>[6x]TLGTGNNGAKTEINKDGLTITPANGAGANNANTISVTKDGISAGGQSVKNVV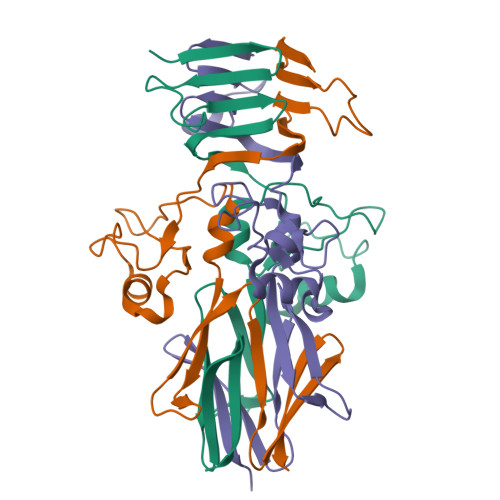SGLKKFGDANFDPLTSSADNLTKQNDDAYKGLTNLDEKGTDKQTPVVADNTAATVGDLRGLGWVISADKTTGGSTEYHDQVRNANEVKFKSGNGINVSGKTVNGRREITFELAKGEVVKSNE> MPEARTSTPRERYRTQVRAEIKDHAWEQIATAGASALSLNAIAKRMGMSGPALYRYFDGRDELITELIRDAYRSQADSLRAAAASGADLAGLAHALRAWALDDPQRYFLIFGTPVPGYRAPDDITEIAAETMAVIVDACAALPPSDGTDGAFDAHLDTHRQWAGDRPAPSSALHRALSFWSRLHGVL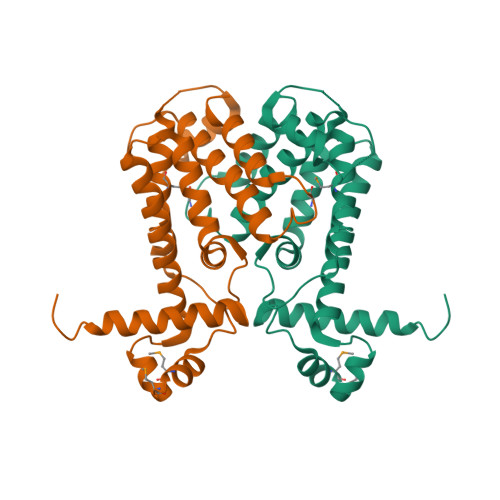SLELAGQFTGMGFDSALLFEAELKDLLGP>[2x]DCNILQRLKVKMQWAKAYGFGTERAKFGNSLWTSIFNYAPDARDLFKSVKSEDMRSPQFKAHIARVIGGLDRVISMFDNEDALNADLEHLKSQHDPRGLDALNFVVFGKALFATVGGQFGVCFDLPAWESCYKVIAMGITGNDMFS;>SECGPLQRLKVKRQWAEAYGSGNGREEFGHFIWANVFKVAPSARDMFKRVRGDNIYTPAFRAHATRVLGGLDMCVALLDDESVLNTQLAHLASQH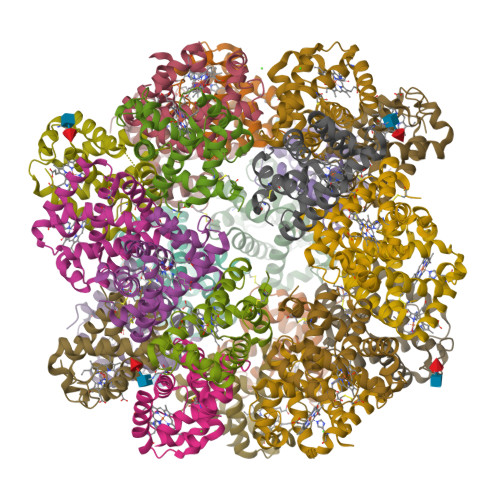SSRGVSAEQYNVVEHAVMMGVEHEIGQNVFDKDAWQACLDVITSGIQGN[2x];>SSNSCTTEDRREMQLMWANVWSAQFTGRRLAIAQAVFKDLFAHVPDAVGLFDRVHGTEIDSSEFKAHCIRVVNGLDSAIGLLSDPSTLNEQLSHLATQHQERAGVTKGGFSAIAQSFLRVMPQVASCFNPDAWSRCFNRITNGMTEGLAE[2x];>[2x]SEFCSEADATIVIKQWNQIYNAGIGAKSRWTMGNEIFSSLFKLKPESEVLFNNVNVANMSSGAFHAHTVRVLSGLDMGINYLNDAGTLTSLTAHLAAQHVARTGLKAVYFDAMGKVLMTVLPSLIDNFNPDAWRNCLLPLKNAIAKGLP>[4x]FACKTANGTAIPIGGGSANVYVNLAPVVNVGQN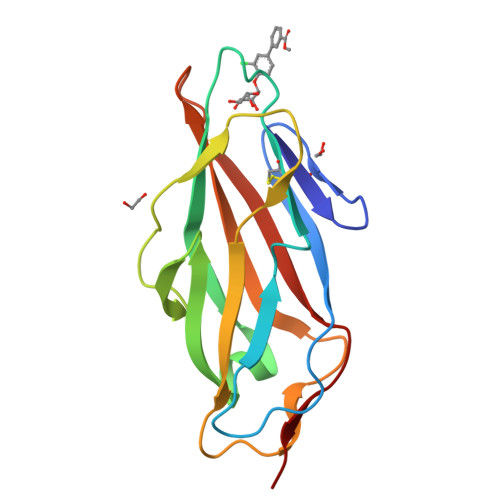LVVDLSTQIFCHNDYPETITDYVTLQRGSAYGGVLSNFSGTVKYSGSSYPFPTTSETPRVVYNSATDKPWPVALYLTPVSSAGGVAIKAGSLIAVLILRQTNNYNSDDFQFVWNIYANNDVVVPT>[6x]MAENLNLFTSTQEVVKEALNKLGYDEAMYELLKEPLRLLKVRIPVKMDDGTTQVFTGYRAQHSDAVGPTKGGVRFHPMVSEDEVKALSMWMTLKCGIVDLPYGGGKGGIICDPRQMSMGELERLSRGYVRAISQIVGPTKDIPGPDMFTNAQIMAWMMDEYSRMDEFNSPGFITGKPLVLGGSKGRDRATAEGVTIVIQEAAKKRNIDIKGARVVIQGFGNAGSFLAK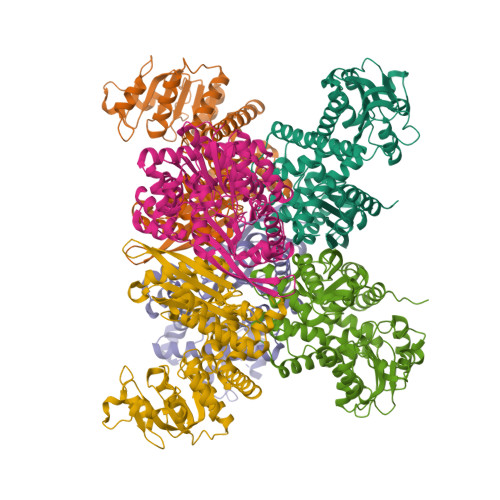FMSDLGAKVIGISDAYGALHDPNGLDIDYLLDRRDSFGTVTTLFENTITNQELLELDCDILVPAAIENQITAENAHNIKATIVVEAANGPTTSEATKILTERGILLVPDVLASAGGATVSYFEWVQNNMGYYWEEEEVQEKLYKKMYDSFEAVYTTATTRNIDMRLAAYMVGVRRTAEASRFRGWVLEHHHHHH> D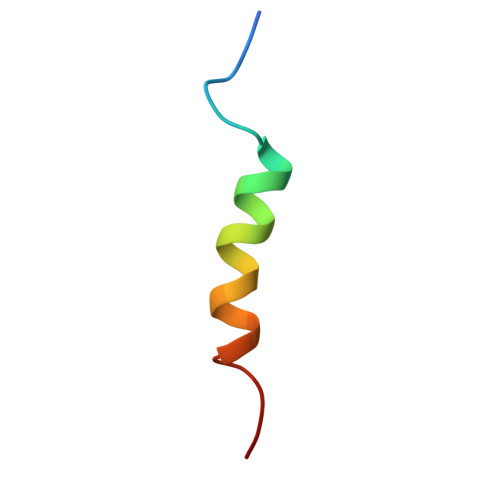DDLGFDPFVETQKGLAELMENEVVQ> AMALEARLEQASILKKVVDAIKDLVQDCNFDCNDSGIALQAMDNSHVALVSMMLKAEGFSPYRCDRNIALGVNLTSLTKVLRAAQNEDILTLKAEDAPDVLNLVFESSETDRISEYDLKLMDIDQEHL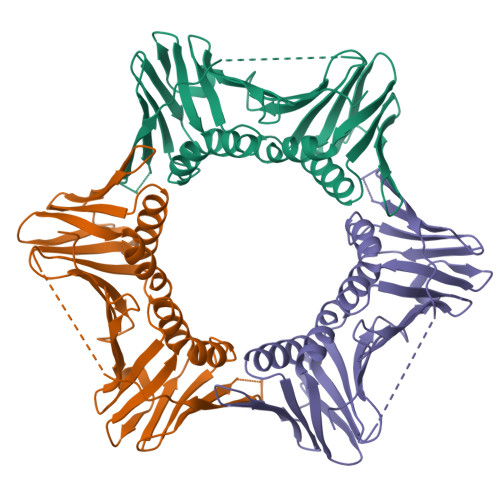GIPETEYAATITMPSNEFKRITTDLMAMSESVTIEANKDGVKFSCQGDIGNGSVTLRQHTNVEKPNESIEIELSEPVSLTFSLKYLVNFCKASALSNTVKICLSNEVPLLVEYSLGGSSYLRFYLAPKIGDDE> DLYFNPRFLADDPQAVADLSRFENGQELPPGTYRVDIYLNNGYMATRDVTFNTGDSEQGIVPCLTRAQLASMGLNTASVAGMNLLADDACVPLTTMVQDATAHLDVGQQRLNLTIPQAFMSNRARGYIPPELWDPGINAGLLNYNFSGNSVQNRIGGNSHYAYLNLQSGLNIGAWRLRDNTTWSYNSSDRSSGSKNKWQHINTWLERDIIPLRSRLTLGDGYTQGDIFDGINFRGAQLASDDNMLPDSQRGFAPVIHGIARGTAQVTIKQNGYDIYNSTVPPGPFTINDIYAAGNSGDLQVTIKEADGSTQIFTVPYSSVPLLQREGHTRYSITAGEYRSGNAQQEKPRFFQSTLLHGLPAGWTIYGGTQLADRYRAFNFGIGKNMGALGALSVDMTQANSTLPDDSQHDGQS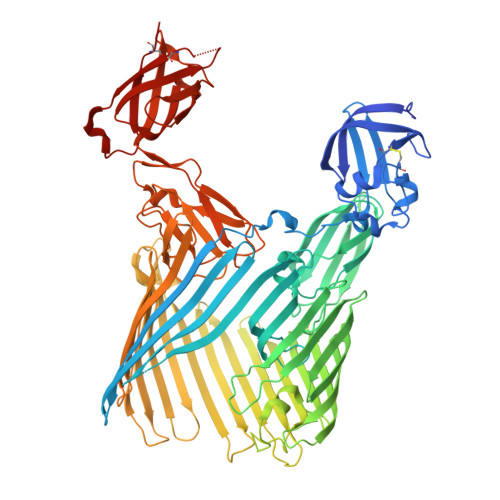VRFLYNKSLNESGTNIQLVGYRYSTSGYFNFADTTYSRMNGYNIETQDGVIQVKPKFTDYYNLAYNKRGKLQLTVTQQLGRTSTLYLSGSHQTYWGTSNVDEQFQAGLNTAFEDINWTLSYSLTKNAWQKGRDQMLALNVNIPFSHWLRSDSKSQWRHASASYSMSHDLNGRMTNLAGVYGTLLEDNNLSYSVQTGYAGGGDGNSGSTGYATLNYRGGYGNANIGYSHSDDIKQLYYGVSGGVLAHANGVTLGQPLNDTVVLVKAPGAKDAKVENQTGVRTDWRGYAVLPYATEYRENRVALDTNTLADNVDLDNAVANVVPTRGAIVRAEFKARVGIKLLMTLTHNNKPLPFGAMVTSESSQSSGIVADNGQVYLSGMPLAGKVQVKWGEEENAHCVANYQLPPESQQQLLTQLSAECRSAWSHPQFEK>[4x]MLNSFKLSLQYILPKLWLTRLAGWGASKRAGWLTKLVIDLFVKYYKVDMKEAQKPDTASYRTFNEFFVRPLRDEVRPIDTDPNVLVMPADGVISQLGKIEEDKILQAKGHNYSLEALLAGNYLMADLFRNGTFVTTYLSPRDYHRVHMPCNGILREMIYVPGDLFSVNHLTAQNVPNLFARNERVICLFDTEFGPMAQILVGATIVGSIETVWAGTITPPREGIIKRWTWPAGENDGSVALLKGQEMGRFKLG;>[4x]XTVINLFAPGKVNLVEQLESLSVTKIGQPLAVSTGHHHHHHG

Phosphatidylethanolamine (PE), a major component of the cellular membrane across all domains of life, is synthesized exclusively by membrane-anchored phosphatidylserine decarboxylase (PSD) in most bacteria. PSD is translated as an inactive proenzyme and undergoes self-cleavage between a conserved Gly-Ser pair to become an active αβ-heterodimer. This maturation step results in the post-translational modification of the N-terminus serine to pyruvoyl in the α-subunit, which is an indispensable prosthetic group for decarboxylation activity. After the proenzyme undergoes auto-proteolysis, an active complex is formed between the α- and β-chains, which are mainly responsible for catalytic activity and membrane association, respectively.

Using native and selenomethionine-derivatized recombinant PSD1–287, the crystal structures of apo PSD1–287 were determined from two crystal forms at resolutions of 1.90 and 2.63 Å, which are described as Apo-PSD1 and Apo-PSD2, respectively. The asymmetric unit of Apo-PSD1 contains two αβ-heterodimers, whereas that of Apo-PSD2 contains four. No detergent molecules were modeled in Apo-PSD2 structure. The N-terminal pyruvoyl residue (Pvl-254) of the α-subunit was unambiguously identified in both apo structures. Gly-253 of the β subunit, which is no longer connected to Pvl-254 after auto-cleavage, is approximately 12.6 Å apart when the distance between two Cαs is measured, and it forms a salt bridge with the side chain of Arg-221. Consequently, Pvl-254, which is located at the base of the funnel-shaped active site, is open for substrate binding. The biological assembly of PSD1–287 appears to be a dimer of αβ-heterodimers, (αβ)2, which is commonly identified in all four structures presented herein.>[6x]SNANSYVALYKFLPQENNDLALQPGDRIMLVDDSNEDWWKGKIGDRVGFFPANFVQRVRPGENVWRCCQPFSGNKEQGYMSLKENQICVGVGRSKDADG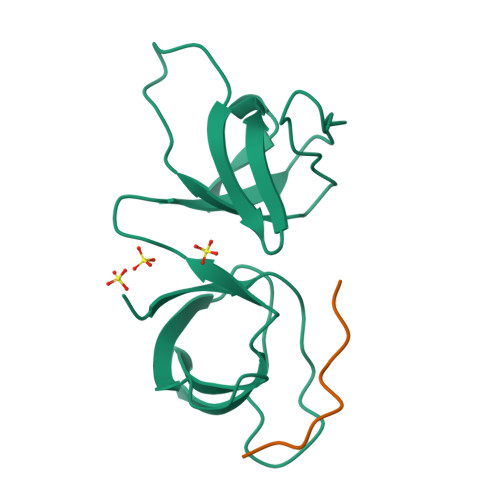FIRVSSGKKRGLVPVDALTEI;>EDEPEIPLSPRPRP[6x]>MATVEPETTPTPNPPTTEEEKTESNQEVANPEHYIKHPLQNRWALWFFKNDKSKTWQANLRLISKFDTVEDFWALYNHIQLSSNLMPGCDYSLFKDGIEPMWEDEKNKRGGRWLITLNKQQRRSDLDRFWLETLLCLIGESFDDYSDDVCGAVVNVR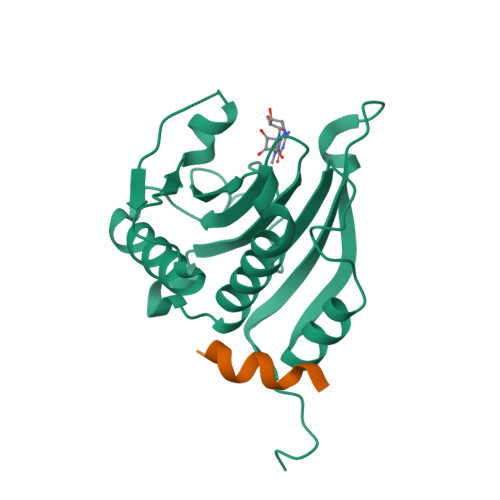AKGDKIAIWTTECENREAVTHIGRVYKERLGLPPKIVIGYQSHADTATKSGSTTKNRFVV[2x];>RIIYDRKFLMECRN[2x]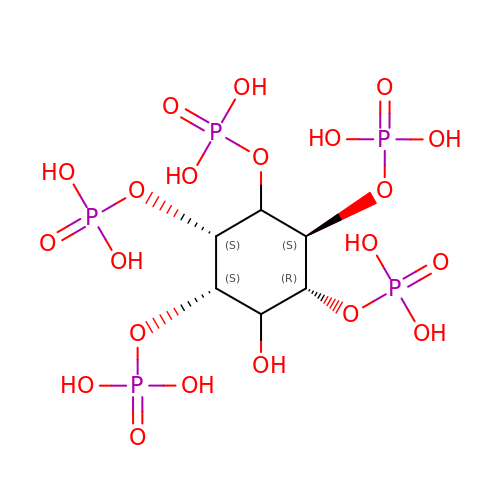(1R,2S,3R,4S,5S,6R)-6-HYDROXYCYCLOHEXANE-1,2,3,4,5-PENTAYL PENTAKIS[DIHYDROGEN (PHOSPHATE)] | C6 H17 O21 P5 | CTPQAXVNYGZUAJ-PTQMNWPWSA-N>GPLGSVQMLISFTSFNDESGENAEKLLQFKRWFWSIVEKMSMTERQDLVYFWTSSPSLPASEEGFQPMPSITIRPPDDQHLPTANTCISRLYVPLYSSKQILKQKLLLAIKTKNFGFV[2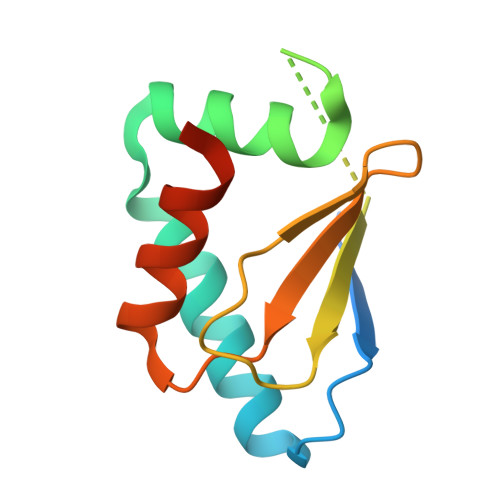x]2-[2-(2-ethoxyethoxy)ethoxy]ethanol | C8 H18 O4 | 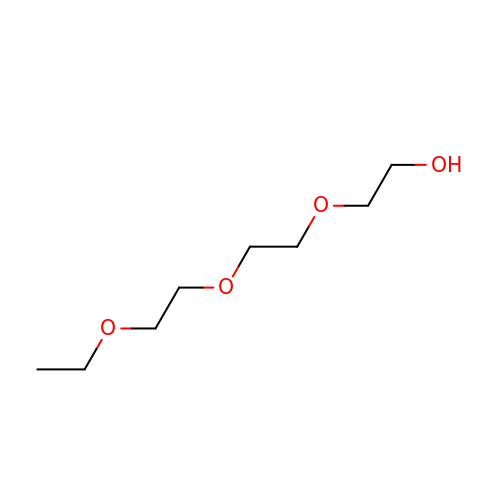WFSMVVDJSNMRAR-UHFFFAOYSA-N6-[(cyclopentylmethyl)amino]pyridine-3-carboxamide 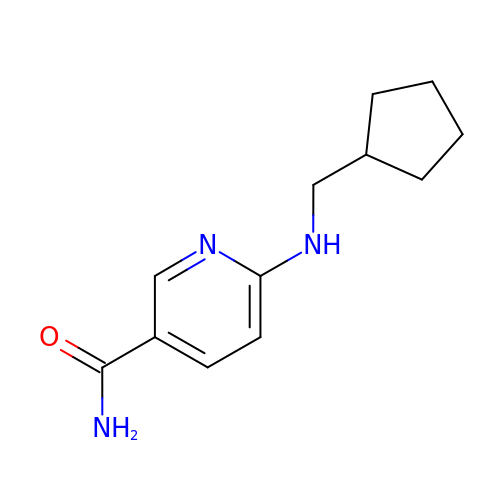| C12 H17 N3 O | KSUTVZCNRWWYFG-UHFFFAOYSA-N> SKFLDRFRYFKQKGETFADGHGQLLNTNRDWEDGYRQRWQHDKIVRSTHGVNCTGSCSWKIYVKNGLVTWETQQTDYPRTRPDLPNHEPRGCPRGASYSWYLYSANRLKYPMMRKRLMKMWREAKALHSDPVEAWASIIEDADKAKSFKQARGRGGFVRSSWQEVNELIAASNVYTIKNYGPDRVAGFSPIPAMSMVSYASGARYLSLIGGTCLSFYDWYCDLPPASPQTWGEQTDVPESADWYNSSYIIAWGSNVPQTRTPDAHFFTEVRYKGTKTVAVTPDYAEIAKLCDLWLAPKQGTDAAMALAMGHVMLREFHLDNPSQYFTDYVRRYTDMPMLVMLEERDGYYAAGRMLRAADLVDALGQENNPEWKTVAFNTNGEMVAPNGSIGFRWGEKGKWNLEQRDGKTGEETELQLSLLGSQDEIAEVGFPYFGGDGTEHFNKVELENVLLHKLPVKRLQLADGSTALVTTVYDLTLANYGLERGLNDVNCATSYDDVKAYTPAWAEQITGVSRSQIIRIAREFADNADKTHGRSMIIVGAGLNHWYHLDMNYRGLINMLIFCGCVGQSGGGWAHYVGQEKLRPQTGWQPLAFALDWQRPARHMNSTSYFYNHSSQWRYETVTAEELLSPMADKSRYTGHLIDFNVRAERMGWLPSAPQLGTNPLTIAGEAEKAGMNPVDYTVKSLKEGSIRFAAEQPENGKNHPRNLFIWRSNLLGSSGKGHEFMLKYLLGTEHGIQGKDLGQQGGVKPEEVDWQDNGLEGKLDLVVTLDFRLSSTCLYSDIILPTATWYEKDDMNTSDMHPFIHPLSAAVDPAWEAKSDWEIYKAIAKKFSEVCVGHLGKETDIVTLPIQHDSAAELAQPLDVKDWKKGECDLIPGKTAPHIMVVERDYPATYERFTSIGPLMEKIGNGGKGIAWNTQSEMDLLRKLNYTKAEGPAKGQPMLNTAIDAAEMILTLAPETNGQVAVKAWAALSEFTGRDHTHLALNKEDEKIRFRDIQAQPRKIISSPTWSGLEDEHVSYNAGYTNVHELIPWRTLSGRQQLYQDHQWMRDFGESLLVYRPPIDTRSVKEVIGQKSNGNQEKALNFLTPHQKWGIHSTYSDNLLMLTLGRGGPVVWLSEADAKDLGIADNDWIEVFNSNGALTARAVVSQRVPAGMTMMYHAQERIVNLPGSEITQQRGGIHNSVTRITPKPTHMIGGYAHLAYGFNYYGTVGSNRDEFVVVRKMKNIDWLDGEGNDQVQESVK;> MKIRSQVGMVLNLDKCIGCHTCSVTCKNVWTSREGVEYAWFNNVETKPGQGFPTDWENQEKYKGGWIRKINGKLQPRMGNRAMLLGKIFANPHLPGIDDYYEPFDFDYQNLHTAPEGSKSQPIARPRSLITGERMAKIEKGPNWEDDLGGEFDKLAKDKNFDNIQKAMYSQFENTFMMYLPRLCEHCLNPACVATCPSGAIYKREEDGIVLIDQDKCRGWRMCITGCPYKKIYFNWKSGKSEKCIFCYPRIEAGQPTVCSETCVGRIRYLGVLLYDADAIERAASTENEKDLYQRQLDVFLDPNDPKVIEQAIKDGIPLSVIEAAQQSPVYKMAMEWKLALPLHPEYRTLPMVWYVPPLSPIQSAADAGELGSNGILPDVESLRIPVQYLANLLTAGDTKPVL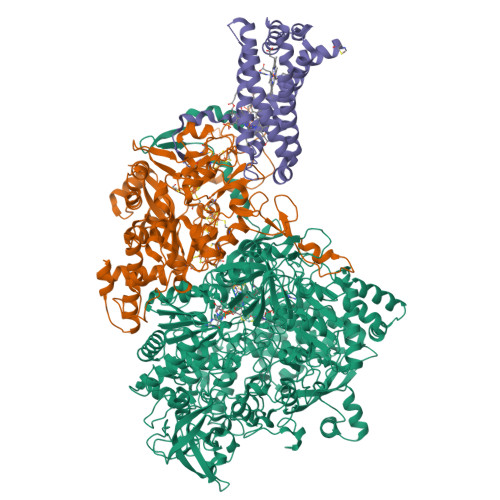RALKRMLAMRHYKRAETVDGKVDTRALEEVGLTEAQAQEMYRYLAIANYEDRFVVPSSHRELAREAFPEKNGCGFTFGDGCHGSDTKFNLFNSRRIDAIDVTSKTEPHP;> MQFLNMFFFDIYPYIAGAVFLIGSWLRYDYGQYTWRAASSQMLDRKGMNLASNLFHIGILGIFVGHFFGMLTPHWMYEAWLPIEVAQKMAMFAGGASGVLCLIGGVLLLKRRLFSPRVRATTTGADILILSLLVIQCALGLLTIPFSAQHMDGSEMMKLVGWAQSVVTFHGGASQHLDGVAFIFRLHLVLGMTLFLLFPFSRLIHIWSVPVEYLTRKYQLVRARH> MAGGKLTPRQKMINLMYLVF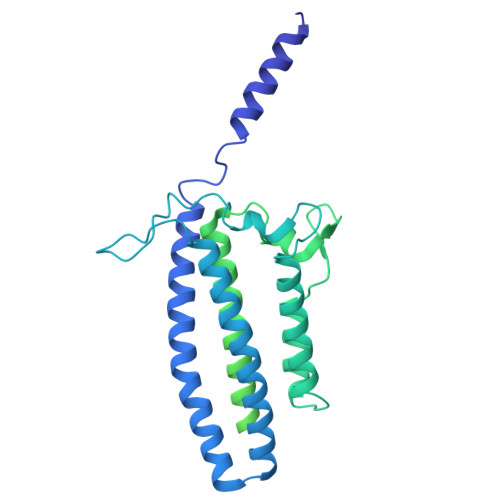IAMLAMNVSKEVISAFGLMNEKFEAANTSSVTTNESLLTSLDQKAAEAKGEFAKAAETAHKVQAASKEFYDYIGTLKTQAVKGFEVDKETGKMPYEAMDRGDNIDDWFTGDGYTKKGNEIIAKIEKYKSDIKAALGTDKKYAGIISEVEKKFDVSDVKNKEGIKEKYLAYHFKGFPAIASAAKLSAWQNDVKKTEADVYNSALGKAAVAAASYSNYQAIVVLDKNAYFQGEKVTGKVVLGRYDENTKPTSFQGPGQIVNGQAVISLTAGGVGEQDINGQFTFLEDGKNIPLKFSGKYVVVPRPNSATISADKMNVVYRGVVNPISVSFAGVDANKIVASAPGLSSAGKPGKYNMSPGQGTEATISVTGTLPNGDKVTDKKTFRIKGIPGPTGTIRGEMGVVKGPKSNLEIATIGAKLLDFDFEVGLDVVGFNMKIAGQPTVVVTGNKMNAQCKSVLARAGKGDQVTISEIKTKLVGAGSYLLPRTAPVIYEIQ> GPLGSTAFRKFYERGDFPIALEHDSKGNKIAWKVEIEKLDYHHYLPLFFDGLCEMTFPYEFFARQGIHDMLEHGGNKILPVLPQLIIPIKNALNLRNRQVICVTLKVL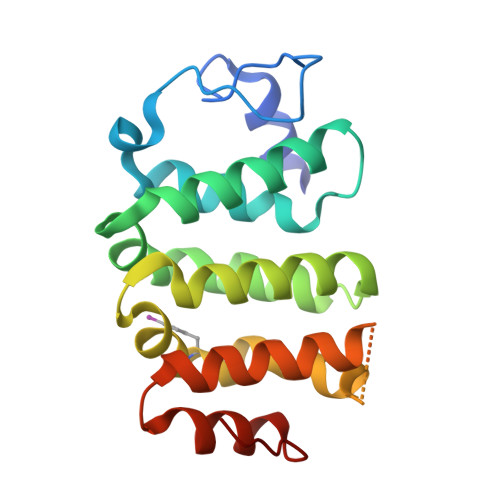QHLVVSAEMVGKALVPFYRQILPVLNIFKNMNVNSGDGIDYSQQKRENIGDLIQETLEAFERYGGENAFINIKYVVPTYESCLLN> GSMDFPYDLNALFPERISVLDSNLSAGRKAHGRPDPLPQVTTVIDELGKASSKAQQLPAPITSAAKLQAN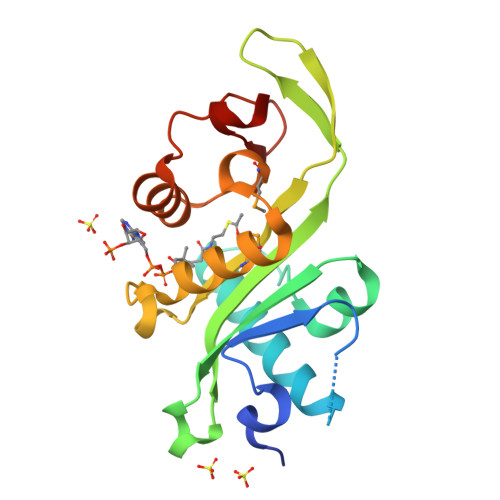RHHLYLLKDGEQNGGRGVIVGFLKVGYKKLFLLDQRGAHLETEPLCVLDFYVTETLQRHGYGSELFDFMLKHKQVEPAQMAYDRPSPKFLSFLEKRYDLRNSVPQVNNFVVFAGFFQSRSG> RQTPEPSGRKPRKDSTGLLRYCVQKHDASRLHYDFRLELDGTLKSWAVPKGPCLDPAVKRLAVQVEDHPLDYADFEGSIPQGHYGAGDVIVWDRGAWTPLDDPREGLEKGHL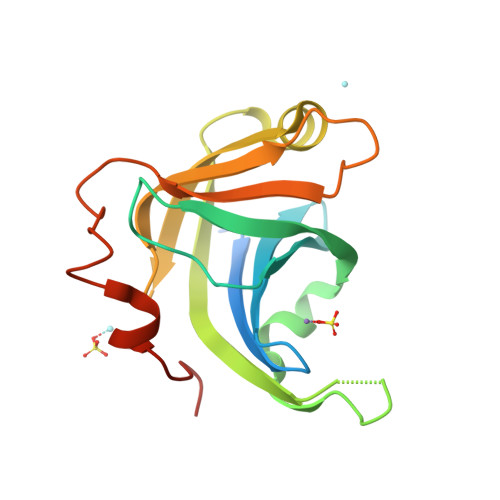SFALDGEKLSGRWHLIRTNLRGKQSQWFLVKAKDGEARSLDRFDVLKERPDSVLSERTL>[4x]MKVGIVGSGMVGSATAYALALLGVAREVVLVDLDRKLAQAHAEDILHATPFAHPVWVRAGSYGDLEGARAVVLAAGVAQRPGETRLQLLDRNAQVFAQVVPRVLEAAPEAVLLVATNPVDVMTQVAYRLSGLPPGRVVGSGTILDTARFRALLAEYLRVAPQSVHAYVLGEHGDSEVLVWSSAQVGGVPLLEFAEARGRALSPEDRARI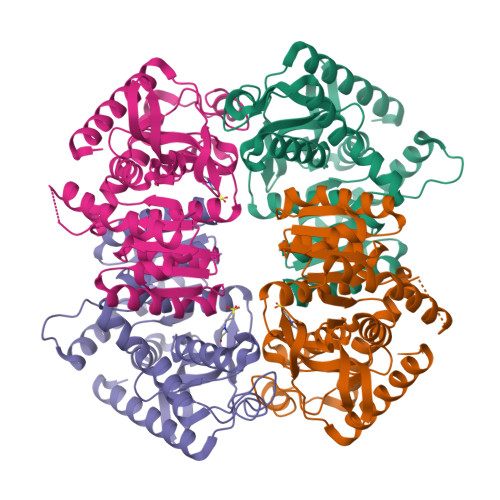DEGVRRAAYRIIEGKGATYYGIGAGLARLVRAILTDEKGVYTVSAFTPEVEGVLEVSLSLPRILGAGGVEGTVYPSLSPEEREALRRSAEILKEAAFALGF>MALNSINTNA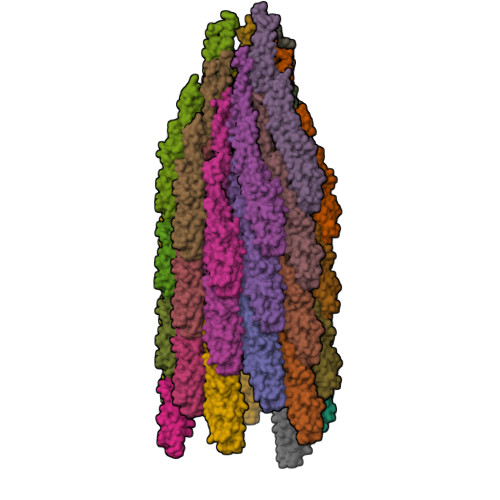GAMIALQNLNGTNSELTTVQQRINTGKKIASAKDNGAIWATAKNQSATAASMNAVKDSLQRGQSTIDVALAAGDTITDLLGKMKEKALAASDTSLNTASFNALKSDFDSLRDQIEKAATNAKFNGVSIADGSTTKLTFLANSDGSGFTVNAKTISLAGIGLTTTSTFTTAAAAKTMIGTIDTALQTATNKLASLGTSSVGLDTHLTFVGKLQDSLDAGVGNLVDADLAKESAKLQSLQTKQQLGVQALSIANQSSSSILSLFR[36x]>QSVKESEGGLFKPTDTLTLTCTASGFSLNGYGVIWVRQAPGKGLEWIGSAGAYGRIYYPNWARSRATITRNTNLNTVSLKMTSLTAADTATYFCARRTNVSTSVGFDSWGPGTLVTVSSSSGQPKAPSVFPLAPCCGDTPSSTVTLGCLVKGYLPEPVTVTWNSGTLTNGVRTFPSVRQSSGLYSLSSVVSVTSSSQPVTCNVAHPATNTKVDKTVAPSTCSHHHHHH[6x];>[6x]DMTQTPSSKSVPVGDTVTINCQASESVYSNNRLSWFQQKPGQPPKLLIYLVSTLASGVPSRFKGSGSGTQFTLTISDVVCDDAATYYCVGYKSSTTDGLAFGGGTEVVVKGDPVAPTVLIFPPAADQVATGTVTIVCVANKYFPDVTVTWEVDGTTQTTGIENSKTPQNSADCTYNLSSTLTLTSTQYNSHKEYTCKVTQGTTSVVQSFNRGDC;>[6x]RNIIXGSDS

Phosphohistidine (pHis) is a labile posttranslational modification with two isoforms, 1-pHis and 3-pHis, involved in many cellular processes across the kingdoms of life. Previously, we developed monoclonal antibodies (mAbs) against the 1-pHis and 3-pHis modifications using stable phosphotriazolylalanine mimetics as immunogens. Here, we report structures of Fab fragments derived from five rabbit pHis mAbs crystallized in complex with their cognate 1-pTza and 3-pTza peptides. These structures provide critical information about the molecular mechanism of phosphoepitope recognition, isomer specificity, sequence independence, and noncross-reactivity to other phosphoamino acids.

In the 1-pHis Fabs the peptidyl phosphate is oriented toward the CDRH2 loop, whereas it is anchored on CDRH3 in the 3-pHis antibodies thus creating a deeper pocket. The key feature of phosphate binding by the 1-pHis Fabs is the participation of Arg95 in CDRH3 loop in forming salt bridges with the phosphate; this type of phosphate interaction is shared with two phosphate-binding superfamilies, FMN-linked oxidoreductases and PRTase, as well as SH2 and PTB domain-containing proteins that recognize pTyr modifications. The bound peptides adopt a type I β-turn conformation around residues I-1-pTza-GS. Analysis with PyIgClassify shows that the canonical conformations of all of the CDRs in 1-pHis Fabs are the same, and that they share common conformations with CDRH2, CDRL1, and CDRL2 in the 3-pHis Fabs. These two isomer classes of Fabs differ primarily in the conformations of CDRH3 and CDRL3, which also provide the primary contact points for the triazolyl group. However, the direct and water-mediated hydrogen bonds formed with the N3 (N3 equivalent in imidazole ring of His) in 1-pHis Fabs and N2 (N1 equivalent in imidazole ring of His) in 3-pHis Fabs means the topography of the CDR can exclude nonisoform specific substrate binding.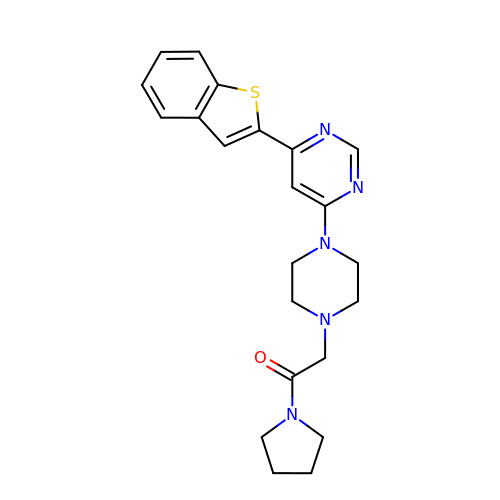4-(1-benzothiophen-2-yl)-6-[4-(2-oxo-2-pyrrolidin-1-ylethyl)piperazin-1-yl]pyrimidine | C22 H25 N5 O S | NDLZMZLRTHDNSQ-UHFFFAOYSA-N>[2x]SNSITENTSWNKEFSAEAVNGVFVLCKSSSKSCATNDLARASKEYLPA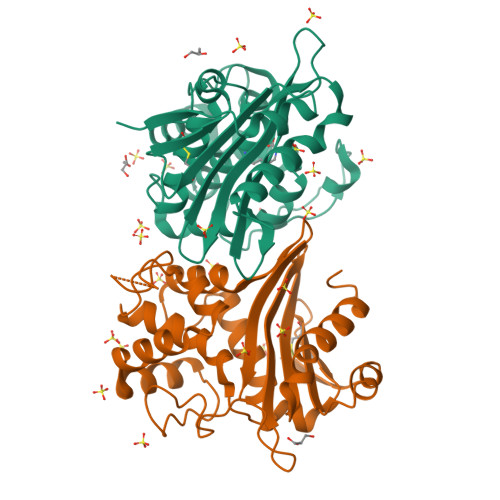STFKIPNAIIGLETGVIKNEHQVFKWDGKPRAMKQWERDLTLRGAIQVSAVPVFQQIAREVGEVRMQKYLKKFSYGNQNISGGIDKFWLEDQLRISAVNQVEFLESLYLNKLSASKENQLIVKEALVTEAAPEYLVHSKTGFSGVGTESNPGVAWWVGWVEKETEVYFFAFNMDIDNESKLPLRKSIPTKIMESEGIIGG2-[1-[(2S)-2-methyl-3-sulfanyl-propanoyl]piperidin-4-yl]ethanamide 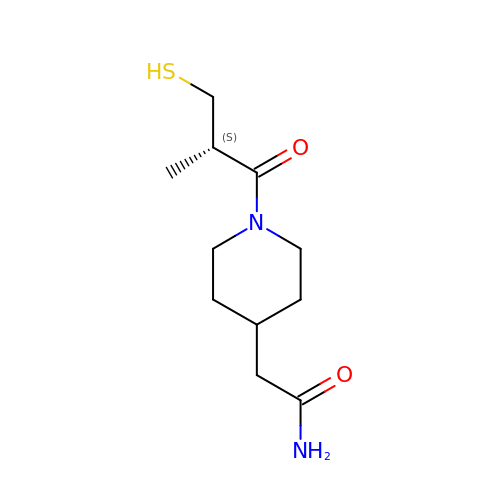| C11 H20 N2 O2 S | MLLZAZRBSAVWPR-MRVPVSSYSA-N> SILDPEVLKVAEYVYQERLSKPYTEVGPEWEYNHKTPYATRATGTGHNLQRFITIDDQRLHRPIHGLAHTMRTLFYSQLMYEAAKRQPHPHRCADGRTIADLSVQDLKKLNIAQL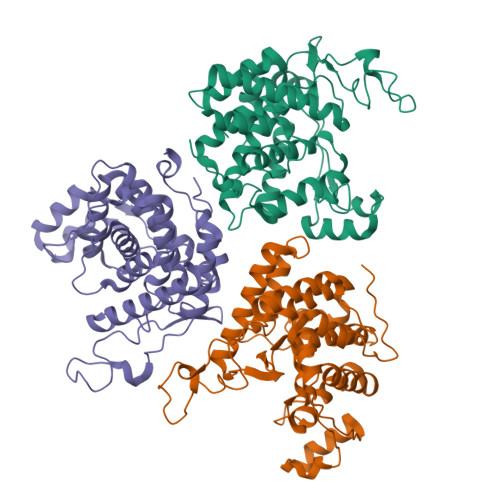FFVAGRESEASYGDAYHRYHLYGAKQFEAYARKHLTHLFSEKEIVLYSRCIEDRIGDRFDETAEGYLIHLSHMIDLMRCKSPVEVFIGHSRGVSGIVPTLIQLFGREDGLDIMHYARSLFAATGEAVPYISSSEWPHLGIESDRVERALKIVGSLEVEGQEADAKKTAQAGFSVDGCYGALVKIDTPDWYHQVKEKEDYDVDEVIALPPQITIREEPPKTNESFLLSL;> GSILDPEVLKVAEYVYQERLSKPYTEVGPEWEYNHKTPYATRATGTGHNLQRFITIDDQRLHRPIHGLAHTMRTLFYSQLMYEAAKRQPHPHRCADGRTIADLSVQDLKKLNIAQLFFVAGRESEASYGDAYHRYHLYGAKQFEAYARKHLTHLFSEKEIVLYSRCIEDRIGDRFDETAEGYLIHLSHMIDLMRCKSPVEVFIGHSRGVSGIVPTLIQLFGREDGLDIMHYARSLFAATGEAVPYISSSEWPHLGIESDRVERALKIVGSLEVEGQEADAKKTAQAGFSVDGCYGALVKIDTPDWYHQVKEKEDYDVDEVIALPPQITIREEPPKTNESFLLSL;> GAMGSILDPEVLKVAEYVYQERLSKPYTEVGPEWEYNHKTPYATRATGTGHNLQRFITIDDQRLHRPIHGLAHTMRTLFYSQLMYEAAKRQPHPHRCADGRTIADLSVQDLKKLNIAQLFFVAGRESEASYGDAYHRYHLYGAKQFEAYARKHLTHLFSEKEIVLYSRCIEDRIGDRFDETAEGYLIHLSHMIDLMRCKSPVEVFIGHSRGVSGIVPTLIQLFGREDGLDIMHYARSLFAATGEAVPYISSSEWPHLGIESDRVERALKIVGSLEVEGQEADAKKTAQAGFSVDGCYGALVKIDTPDWYHQVKEKEDYDVDEVIALPPQITIREEPPKTNESFLLSL> MSIVNILSVNVLNNPAKFSDPYKFEITFECLEPLKSDLEWKLTYVGSA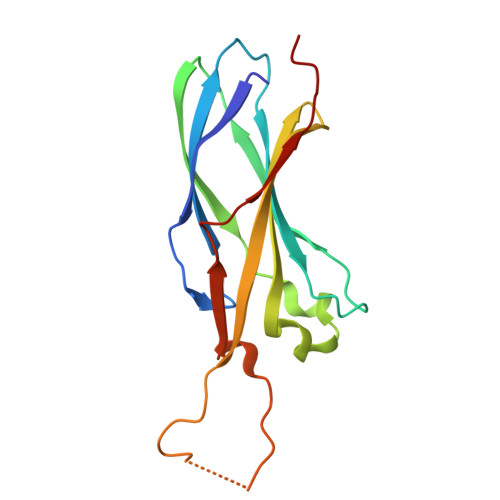TSQSYDQILDTLLVGPIPIGINKFVFEADPPNIDLLPQLSDVLGVTVILLSCAYEDNEFVRVGYYVNNEMEGLNLQEMDDAEIKKVKVDISKVWRSILAEKPRVTRFNIQWDN> MGTFTLHQGQTNLIKSFFRNYYLNAELELPKDMELREFALQPFGSDTYVRHLSFSSSEELRDYLVNRNLPLHLFYSSARYQLPSARNMEEKAWMGSDLLFDIDADHLCKLRSIRFCPVCGNAVVSEKCERDNVETLEYVEMTSECIKRGLEQTRNLVEILEDDFGLKPKVYFSGNRGFHVQVDCYGNCALLDSDERKEIAEYVMGIGVPGYPGGSENAPGWVGRKNRGINGVTIDEQVTIDVKRLIRIPNSLHGKSGLIVKRVPNLDDFEFNETLSPFTGYTIFLPYITIETEVLGSIIKLNRGIPIKIKSSIGIYLHLRNLGEVKAYVR;>MALDVKKYPFIKSLDDELKKYGGGITLTDLLLNSTTLIDQAKDRIQKTKSGDELPHYVSYNEPVLVFYTTLLSLAILNDVKLIRRYAYAEAKQFRSLLHTENEENLLEISKLLDLKINRCDPIKFYLEKKRRIIQKEFCVHFIDYLKYTKDLKEDWKLSGQILHKGYVYLDKNQLIGLIAESIKSKIVEMIRPLNL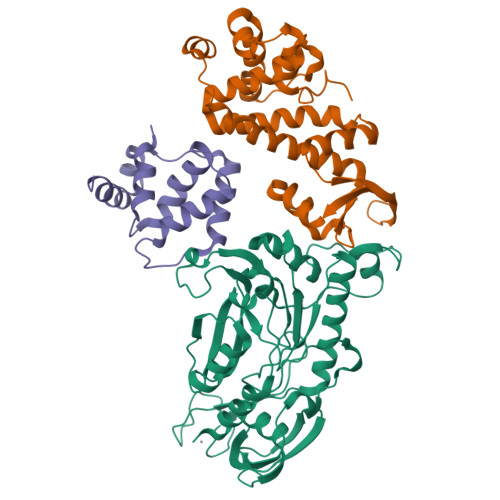KEIPEKLKSLIERRGKVEGKFPPQPKKSSDYSWIEKVLEMGLQDSRKRFILYVASRYLVNVKGVNEDEALQTLKEFYYKLQSGKVYESWLKSVINGVKKKGLLPWSLKRIEERDKEMYNEIIRVLKNS[2x]> EATAGTVTVNAITSDDTIDGIELGQTISISGKAVGGDISVGDVVKMTINNTEYSTTVKAGGIWMIAGVLGSDLAADSEFDVVVTSSDAAGNKVQSIGTSTHSVDLSAEANFSLAEGQQHVLTNLPEGFGFPDGTTEVVTNFGGTITLGD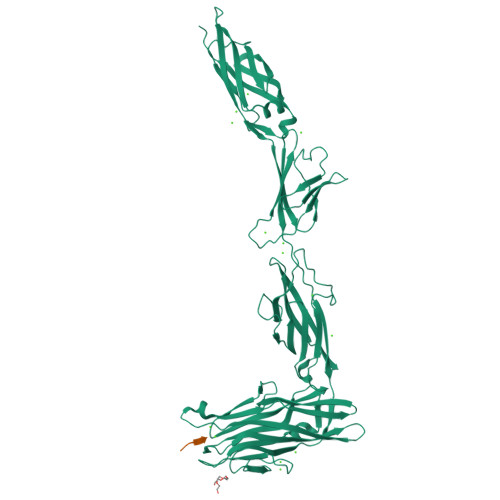DGEYRYDAPVRDHGDAVSDKDSVTVTLEDGRTFTVNLDIQDSAPVAVDDQDSIVVQHEEFEVSEIAASWVSYTHGESVTTFDGTSDLGGVDNDSAKDQIRWGNPAESKQSGYGFIDNDSNLEGRFDLNQDISVGTFTHYNYPVYSGGAITSAEMSVEFSVLDHLGVSTPVTLTVNFDHNETPNTNDVNASRDIVTVQNTHVTFERDGDIYTVQIVGFREVGNPDGEVVTSIYTNENAATSYELVVRVVEGDGYSLPSTEGNIFDDNGLGADSLGADGSVTVVGVAVGAIVSSNESVGHSIEGQYGNLVLNSDGSYVYDVTASVSDIPAGATESFAYLIQDQDGSTSSANLSINVGTN;> DSTD2-[2-chloro-4-(methylsulfonyl)benzoyl]cyclohexane-1,3-dione 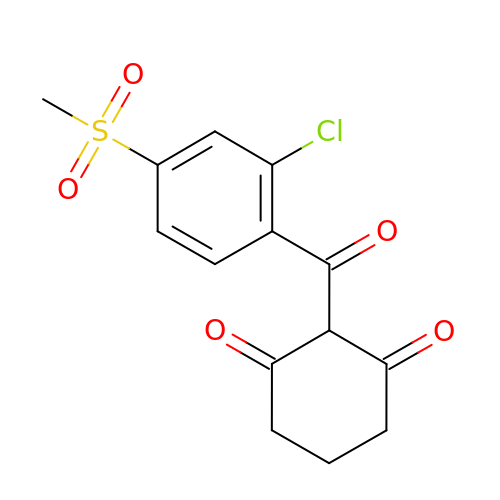| C14 H13 Cl O5 S | PQTBTIFWAXVEPB-UHFFFAOYSA-N> XPDGDRGPRG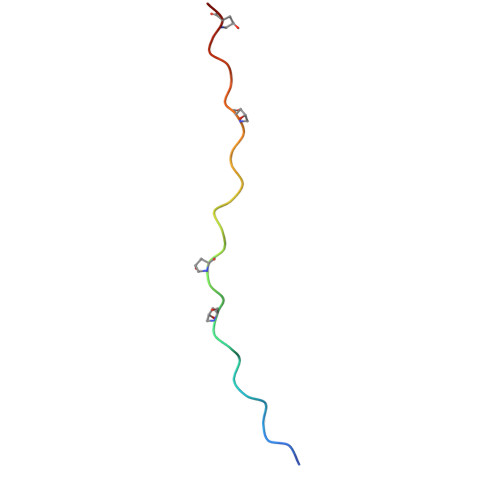PPGYPGDDGPEGDPGPPGDPGX>FTSTFYELFPKTFPKKLPIWTIDQSRLRKEYRQLQAQHHPDMAQQGSEQSSTLNQAYHTLKDPLRRSQYMLKLLRNIDLTQEQTSNEVTTSDPQLLLKVLDIHDELSQMDDEAGVKLLEKQNKERIQDIEAQLGQCYN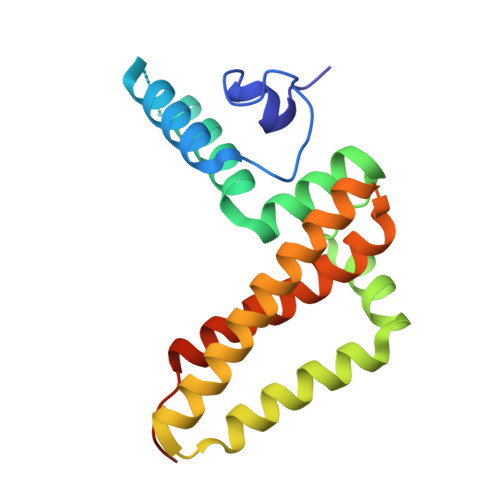DKDYAAAVKLTVELKYWYNLAKAFKDWAPGKQLEMNH[2x]> VSKLWVPNTDFDVAANWSQNRTPCAGGAVEFPADKMVSVLVQEGHAVSDMLLPLDGELVLASGAGFGVSDVGSHLDCGAGEPAVFRDSDRFSWHDPHLWRSGDEAPGLFFVDAERVPCRHDDVFFPPSASFRVGLGPGASPVRVRSISALGRTFTRDEDLAVFLASRAGRLRFHGPGALSVGPEDCADPSGCVCGNAEAQPWICAALLQPLGGRCPQAACHSALRPQGQCCDLCGAVVLLTHGPAFDLERYRARILDTFLGLPQYHGLQVAVSKVPRSSRLREADTEIQVVLVENGPETGGAGRLARALLADVAENGEALGV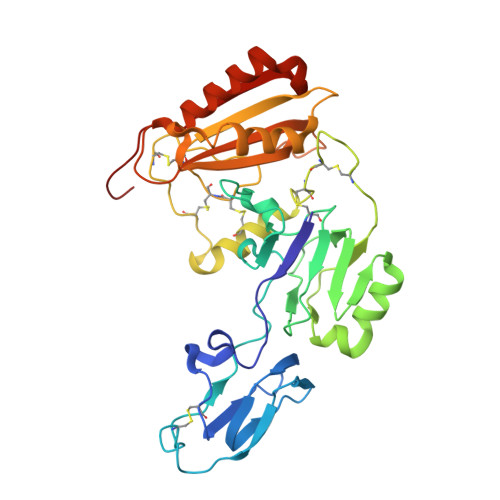LEATMRESGAHVWGSS> EVDKRREINNEHPLLMMPLYANGEEFNQGKYTFWGGDTLTGKWENIPDDLKPYTVIQLHPDDLPKRDGAARDFYEHMLEEAAKYVNPKTGKNEPIPVILTVYTAGNMPYYTSAHWLSTSWIDKMYQKYPNLHGIFSTESYWIWANDIENKAADYLKVSAKNGGYFIWAEQNVGSAIEKA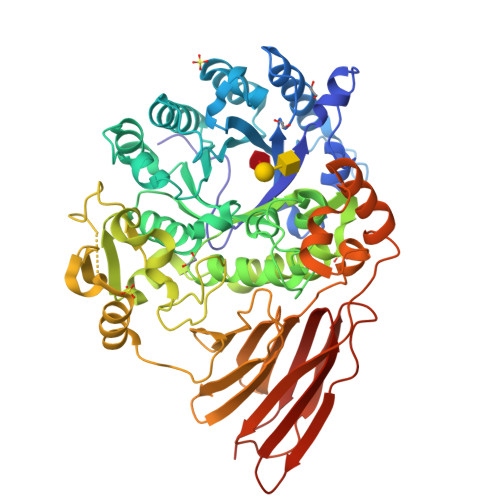FGKNGKIAFQKSVDKYWKNLIFMFKNTPAAEGNDSTTESYMKGLWLSNHTYQWGGLMDTWKWYETGKWKLFASGNIGKSQGDRQWLTEPESMLGEEALGVYLNGGVVYNFEHPAYTYGVNNKESLLFSEVIKEFFRYVIAHPAPSKEKVLEDTKVFIHGDYSNKGNGKFFVNVNTDREQTPLYMTGRYNVIPAIPGVLKTDKLKESVSSSRIQIKEITSPEFSSTQARKEYLNKLYPMNYEGDIFAQKLDNRWFVYNYKVNENVKQTGKLKFNSLEMNVEFEPHTYGIFERISNGLKVNLNNFRTNKDSLWSNAQDANQAKKLPQLTKKGAIKWIEEHYIKDTQFGEKRVTKIVLRGIDKLPTIHSLSGTNNSYDQPSLNFDQKNHMVTITINSNGNLEFELHFLEHTRAPPPPPLRSGC>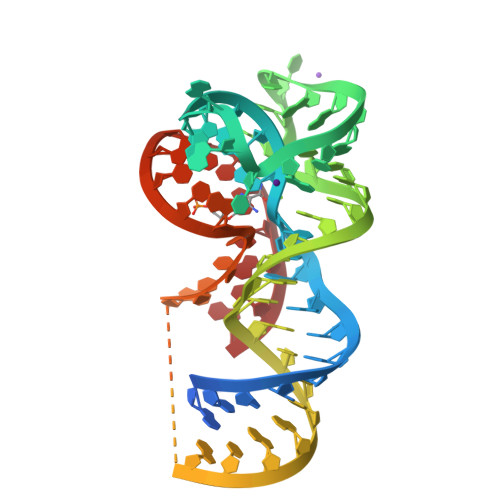[2x]UAUCAGUUAUAUGACUGACGGAACGUGGAAUUAACCACAUGAAGUAUAACGAUGACAAUGCCGACCGUCUGGGCG>SEVGNSQA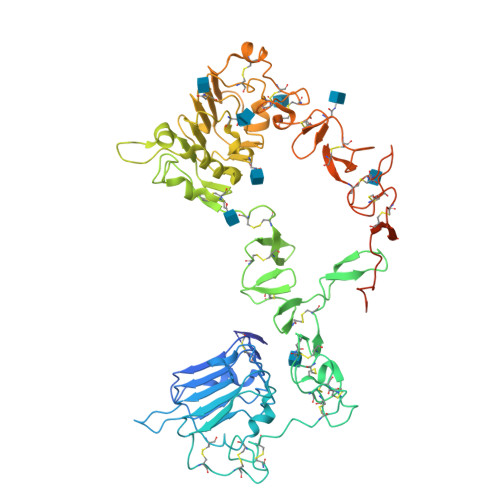VCPGTLNGLSVTGDAENQYQTLYKLYERCEVVMGNLEIVLTGHNADLSFLQWVREVTGYVLVAMNEFSTLPLPNLRVVRGTQVYDGKFAIFVMLNYNTNSSHALRQLRLTQLTEILSGGVYIEKNDKLCHMDTIDWRDIVRDRDAEIVVKDNGRSCPPCHEVCKGRCWGPGSEDCQTLTKTICAPQCNGHCFGPNPNQCCHDECAGGCSGPQDTDCFACRHFNDSGACVPRCPQPLVYNKLTFQLEPNPHTKYQYGGVCVASCPHNFVVDQTSCVRACPPDKMEVDKNGLKMCEPCGGLCPKACEGTGSGSRFQTVDSSNIDGFVNCTKILGNLDFLITGLNGDPWHKIPALDPEKLNVFRTVREITGYLNIQSWPPHMHNFSVFSNLTTIGGRSLYNRGFSLLIMKNLNVTSLGFRSLKEISAGRIYISANRQLCYHHSLNWTKVLRGPTEERLDIKHNRPRRDCVAEGKVCDPLCSSGGCWGPGPGQCLSCRNYSRGGVCVTHCNFLNGEPREFAHEAECFSCHPECQPMEGTATCNGSGSDTCAQCAHFRDGPHCVSSCPHGVLGAKGPIYKYPDVQNECRPCHENCTQGCKGPELQDCLGQTLVLIGKT[2x]>[2x]GAMATAMYLEHYLDSIENLPCELQRNFQ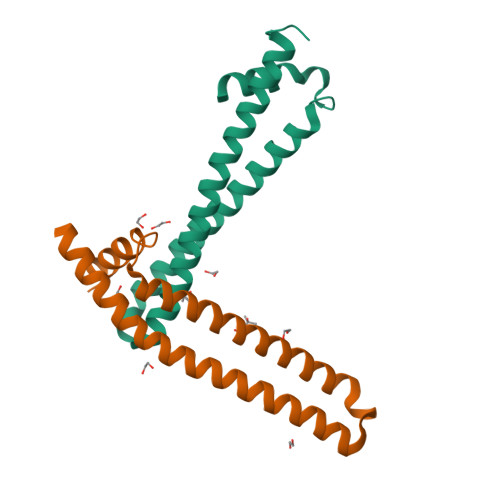LMRELDQRTEDKKAEIDILAAEYISTVKTLSPDQRVERLQKIQNAYSKCKEYSDDKVQLAMQTYEMVDKHIRRLDADLA[(1S,3R,3aR,6aS)-3-(2-azanyl-6-oxidanylidene-1H-purin-9-yl)-5,5-bis(oxidanyl)-1,3,3a,4,6,6a-hexahydrocyclopenta[c]furan-1-yl]methyl 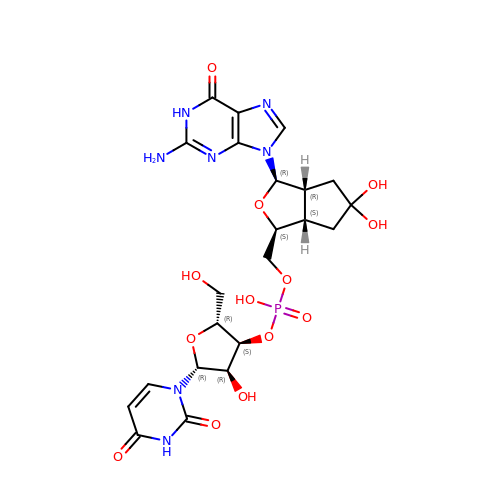[(2R,3S,4R,5R)-5-[2,4-bis(oxidanylidene)pyrimidin-1-yl]-2-(hydroxymethyl)-4-oxidanyl-oxolan-3-yl] hydrogen phosphate | C22 H28 N7 O13 P | UMWHQRFZYGKEGD-MIHJLMQYSA-N FlgA is a periplasmic flagellar protein that chaperones P-ring formation. FlgA possesses a typical signal sequence at its N-terminus, recognized by the Sec-dependent pathway, suggesting that FlgA functions as a P-ring assembly chaperone in the periplasm. P-ring formation is a key step enabling the bacterial flagellum to pass through the outer membrane. FlgA can be divided into three domains, denominated as D1 (residues 1–74), D2 (residues 75–142), and D3 (residues 143–198).

To gain insight into the regulatory mechanism of P-ring assembly by FlgA, two different atomic structures of FlgA from S. enterica, the open and closed forms were solved. Atomic models were built from amino acid residues Q1 through L198 (numbering corresponds to the mature protein) for the open and closed forms and refined at resolutions of 1.95 Å and 2.3 Å, respectively. The conformation of FlgA is different in the two forms. In the closed form, D3 is closer to D1 and forms a compact structure. This occurs largely because of a bend of about 70° around the Cα atom of R136. By studying the 3D structures of FlgA, we identified a pair of residues, R113 and S190, which are within a suitable distance for cross-linking with a disulfide bond that keeps the structure of FlgA in the closed conformation. To understand how the conformational difference between the open and closed forms of FlgA is related to its function, a disulfide bond was engineered by replacing these residues with cysteines (R113C and S190C, respectively). The disulfide bond forces FlgA to stay in the closed form and constrains the movement of domain D3. A rivet structure, which lacks the LP-ring of the hook basal-body, was isolated from the wild-type strain expressing FlgAR113C-S190C. These results indicate that the closed form of FlgA can bind to FlgI, but cannot proceed with subsequent steps, thereby inhibiting FlgI from forming the P-ring. The closed form of FlgA is reminiscent of the PapD structure, an immunoglobulin-like periplasmic chaperone for P pilus biogenesis.

>QDINAQLTTWFSQRLAGFSDEVVVTLRSSPNLLPSCEQPAFSMTGSAKLWGNVNVVARCANEKRYLQVNVQATGNYVAVAAPIARGGKLTPANVTLKRGRLDQLPPRTVLDIRQIQDAVSLRDLAPGQPVQLTMIRQAWRVKAGQRVQVIANGEGFSVNAEGQAMNNAAVAQNARVRMTSGQIVSGTVDSDGNILINLDPNSSSVDKLAAALEHHHHHH[4x]>GDDELYRQSLEIISRYLREQATGAKDTKPMGRSGATSRKALETLRRVGDGVQRNHETAFQGMLRKLDIKNEDDVKSLSRVMIHVFSDGVTNWGRIVTLISFGAFVAKHLKTINQESCIEPLAESITDVLVRTKRDWLVKQRGWDGF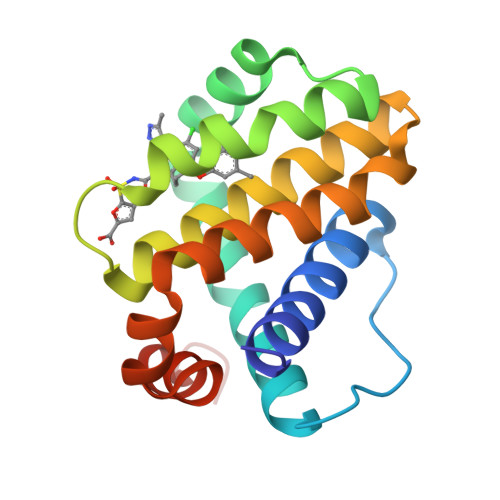VEFFHVEDLEGG[4x]> GSHMQLLTDEEYRELRYGKQETYPLPAGVDALVKDG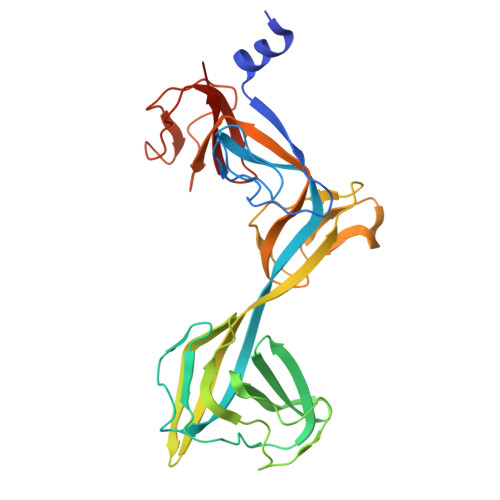EEVVKGQELAPGVVSRMDGVALYRFPRRVRVDYLRKERAALRIPLSAWVEKEAYRPGEVLAELSEPYLFRAEESGVVELKDLAEGHLIYLRQEEEVVARYFLPAGMTPLVVEGEIVEVGQPLAEGKGLLRLPRHMTAKEVEAEEEGDSVHLTLFLEWTEPKDYKVAPHMNVIVPEGAKVQAGEKIVAAIDPEEEVIAEAEGVVHLHEPASILVVKARVYPFEDDVEVTTGDRVAPGDVLADGGKVKSEIYGRVEVDLVRNVVRVVESYDIDAR>GVPRAGKQGQHAVSAYLADARRALGSAGCSQLLAALTAYKQDDDLDKVLAVLAALTTAKPEDFPLLHRFSMFVRPHHKQRFS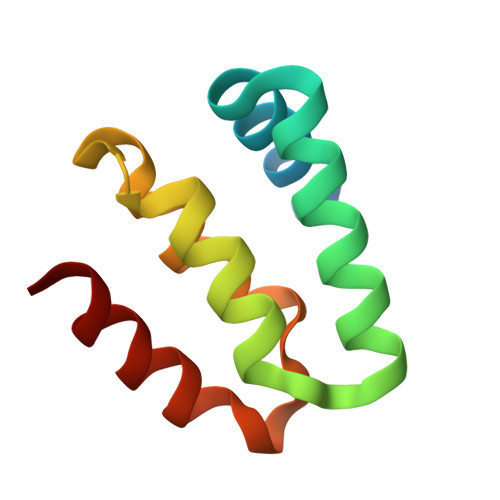QTCTDLTG[7x]> MRRLASPSLRRLQEGQTPHSMRKSAVADARKKIFGYACGMPGEEQWVRPLQGRQMMKWYWPSKYMLQDVQMAQYFQMQAMRFAPRPAHVSLTTLSATMEQCWKKRDAVRAFFQSIDEKVLRENPTLQDLYGLYRTLCPDDPLRTPVDPALWRDPGFTWQHTADQRIVSSSTNREQQGDPSEPAMATRRVAQEQATDKRHISPANINDDVAALLFSRTEQSGAIRNVCAASPYLHGGKNNRSRDRFHNGAREANSSEEDSLEQPKSLILDTESRGTALSRSRTQECLLALSALAETGLGQSASELIQQPVVLRVDIGLGDREPVQDTTAFRKKQEQSRRTLQAALDHDERLARYHGAKHRFFDPLFRRRRLSFLDRFARERIKGEKA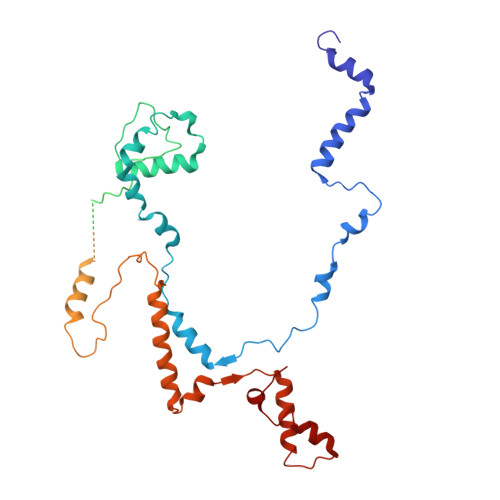RQLGAQLYVKHPDQKPVWP> MRRRYRVVVERDEEGYFVAHVPELHAHTQAQSFEELLRRLQEAIAVSL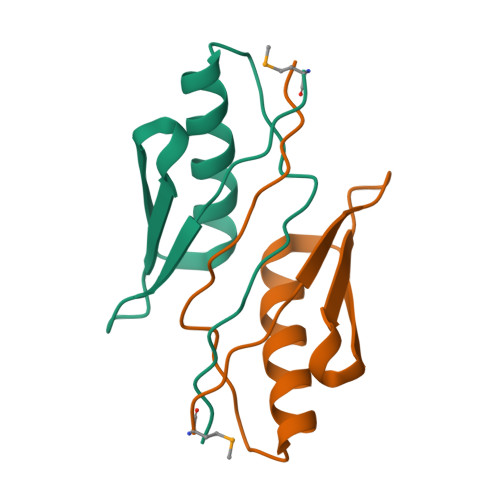EEERAEVVGLEGALEIEAA>[2x]MHGRLKVKTSEEQAEAKRLEREQKLKLYQSATQAVFQKRQAGELDESVLELTSQILGANPDFATLWNCRREVLQHLETEKSPEESAALVKAELGFLESCLRVNPKSYGTWHHRCWLLSRLPEPNWARELELCARFLEADERNF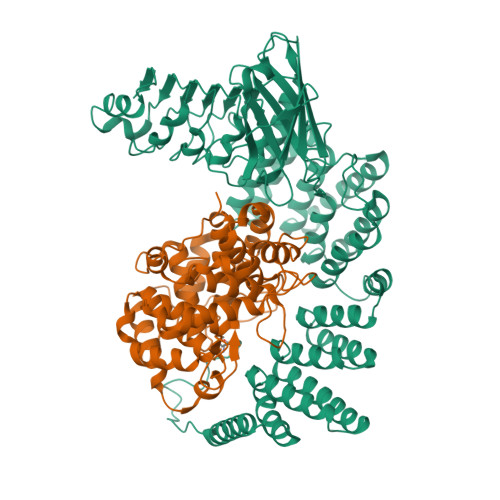HCWDYRRFVAAQAAVAPAEELAFTDSLITRNFSNYSSWHYRSCLLPQLHPQPDSGPQGRLPENVLLKELELVQNAFFTDPNDQSAWFYHRWLLGRAEPHDVLCCVHVSREEACLSVCFSRPLTVGSRMGTLLLMVDEAPLSVEWRTPDGRNRPSHVWLCDLPAASLNDQLPQHTFRVIWTGSDSQKECVLLKDRPECWCRDSATDEQLFRCELSVEKSTVLQSELESCKELQELEPENKWCLLTIILLMRALDPLLYEKETLQYFSTLKAVDPMRAAYLDDLRSKFLLENSVLKMEYADVRVLHLAHKDLTVLCHLEQLLLVTHLDLSHNRLRALPPALAALRCLEVLQASDNALENVDGVANLPRLQELLLCNNRLQQSAAIQPLVSCPRLVLLNLQGNSLCQEEGIQERLAEMLPSVSSILT;>MGTQQKDVTIKSDAPDTLLLEKHADYIASYGSKKDDYEYCMSEYLRMSGVYWGLTVMDLMGQLHRMNKEEILVFIKSCQHECGGVSASIGHDPHLLYTLSAVQILTLYDSIHVINVDKVVAYVQSLQKEDGSFAGDIWGEIDTRFSFCAVATLALLGKLDAINVEKAIEFVLSCMNFDGGFGCRPGSESHAGQIYCCTGFLAITSQLHQVNSDLLGWWLCERQLPSGGLNGRPEKLPDVCYSWWVLASLKIIGRLHWIDREKLRSFILACQDEETGGFADRPGDMVDPFHTLFGIAGLSLLGEEQIKPVSPVFCMPEEVLQRVNVQPELVS[2x]> MAKKTSSKGKLPPGPSPLPVLGNLLQMDRKGLLRSFLRLREKYGDVFTVYLGSRPVVVLCGTDAIREALVDQAEAFSGRGKIAVVDPIFQGYGVIFANGERWRALRRFSLATMRDFGMGKRSVEERIQEEARCLVEELRKSKGALLDNTLLFHSITSNIICSIVFGKRFDYKDPVFLRLLDLFFQSFSLISSFSSQVFELFSGFLKYFPGTHRQIYRNLQEINTFIGQSVEKHRATLDPSNPRDFIDVYLLRMEKDKSDPSSEFHHQNLILTVLSLFAAGTETTSTTLRYGFLLMLKYPHVTERVQKEIEQVIGSHRPPALDDRAKMPYTDAVIHEIQRLGDLIPFGVPHTVTKDTQFRGYVIPKNTEVFPVLSSALHDPRYFETPNTFNPGHFLDANGALKRNEGFMPFSLGK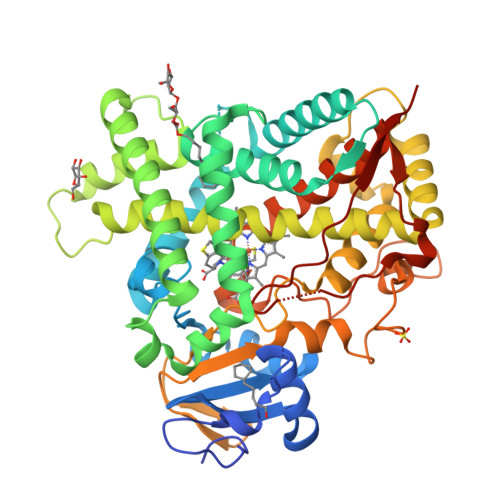RICLGEGIARTELFLFFTTILQNFSIASPVPPEDIDLTPRESGVGNVPPSYQIRFLARHHHHHHH> MESLTLQPIARVDGTINLPGSKSVSNRALLLAALAHGKTVLTNLLDSDDVRHMLNALTALGVSYTLSADRTRCEIIGNGGPLHAEGALELFLGNAGTAMRPLAAALCLGSNDIVLTGEPRMKERPIGHLVDALRLGGAKITYLEQENYPPLRLQGGFT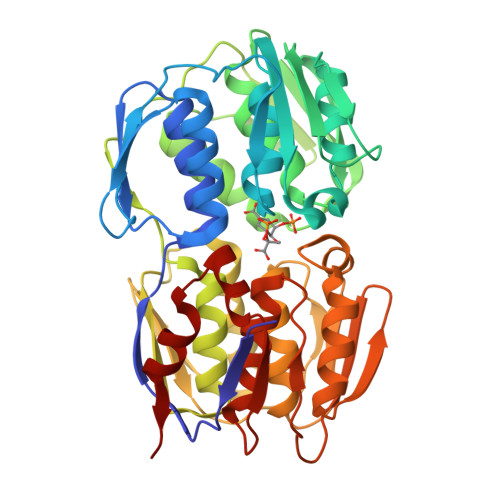GGNVDVDGSVSSQFLTALLMTAPLAPEDTVIRIKGDLVSKPYIDITLNLMKTFGVEIENQHYQQFVVKGGQSYQSPGTYLVEGDASSASYFLAAAAIKGGTVKVTGIGRNSMQGDIRFADVLEKMGATICWGDDYISCTRGELNAIDMDMNHIPAAAMTIATAALFAKGTTTLRNIYNWRVKETDRLFAMATELRKVGAEVEEGHDYIRITPPEKLNFAEIATYNDHRMAMCFSLVALSDTPVTILDPKCTAKTFPDYFEQLARISQAA The ligand-activated transcription factor farnesoid X receptor (FXR, NR1H4)1,2 acting as cellular sensor for bile acids is a crucial metabolic regulator and liver protector. As a member of the nuclear receptor (NR) superfamily it translates ligand signals into changes in gene expression and affects a variety of genes involved in bile acid, glucose and lipid metabolism. NRs share a common architecture of an N-terminal ligand-independent activation domain followed by a DNA-binding domain (DBD), a flexible hinge region and a ligand-binding domain composed of twelve α-helices (α1-α12). Especially the C-terminal α12, the so-called activation function 2 (AF-2) of the LBD, has been identified as crucial for NR activation since stabilisation of α12 and concomitant binding to the core of the LBD provides a surface for co-activator binding.

Structurally, unliganded FXR-LBD comprises the α11 and L:α3-α4 regions in an unordered state and can bind the co-repressor. Superimposition of both spectra, however, revealed significant differences with additional signals and marked CSP. This indicates that the activation function α12 in case of FXR is not disordered and exposed to solvent but even in absence of a ligand is partially stabilised and part of the core LBD. In contrast to the initially proposed mouse trap mechanism and later refined models suggesting an unordered conformation of α12 in solution in absence of an agonist, our results indicate that α12 is ordered and forms part of the core LBD also in absence of a ligand. However, the recruitment of co-activator by the apo-form is not reflected by our NMR studies and might also be a crystallisation artefact. Still, it is possible that the apo-state has a very weak affinity to co-activators that is too low to be captured in our system.

> SHMELTPDQQTLLHFIMDSYNKQRMPQEITNKILKEEFSAEENFLILTEMATNHVQVLVEFTKKLPGFQTLDHEDQIALLKGSAVEAMFLRSAEIFNKKLPSGHSDLLEERIRNSGISDEYITPMFSFYKSIGELKMTQEEYALLTAIVILSPDRQYIKDREAVEKLQEPLLDVLQKLCKIHQPENPQHFACLLGRLTELRTFNHHHAEMLMSWRVNDHKFTPLLCEIWDVQ;> KENALLRYLLDKD> LSNISMSSSEIIDVLCENLNDGIWALRVLYAEGAMNKEKLWDYINQYHKDYQIENEKDYEGKKILPSRYALDIMTARLEGAGLISFKAIGRVRIYDVTDLGNVLIKELEKR;> ISMSSSEIIDVLCENLNDGIWALRVLYAE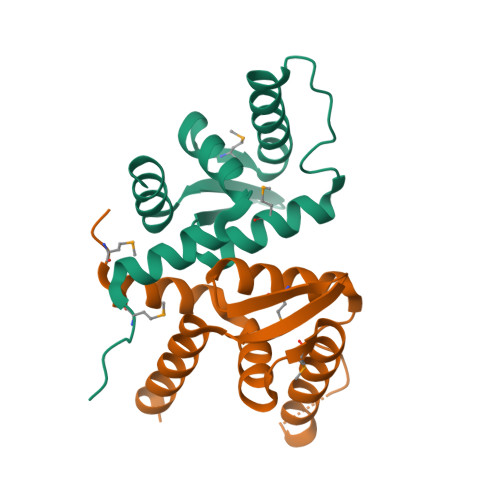GAMNKEKLWDYINQYHKDYQIENEKDYEGKKILPSRYALDIMTARLEGAGLISFKAIGRVRIYDVTDLGNVLIKELEKRVEKNN>SFIKPIYQDINSILIGQKVKRPKSGTLSGHAAGEPFEKLVYKFLKENLSDLTFKQYEYLNDLFMKNPAIIGHEARYKLFNSPTLLFLLSRGKAATENWSIENLFEEKQNDTADILLVKDQFYELLDVKTRNISKSAFAPNIISAYKLAQTCAKMIDNKEFDLFDINYLEVDWELNGEDLVCVSTSFAELFKSEPSELYINWAAAMQIQFHVRDLDQGFNGTREEWAKSYLKHFVTQAEQRAI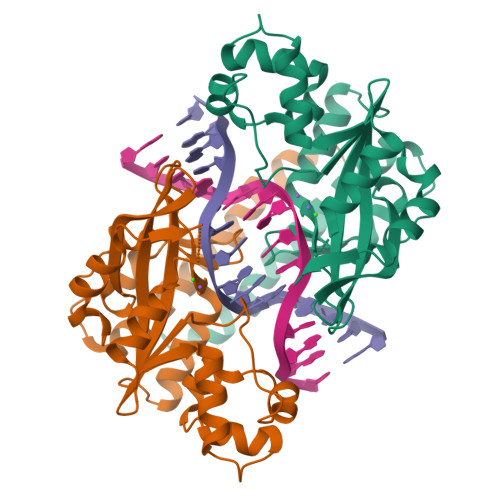SMIDKFVKPFKKYIL[2x]> GSHMAITGTIAAIATAIVPQQGSVGIVRVSGSQAIAIAQTLFDAPGKQVWESHRILYGYIRHPQTRQIVDEALLLLMKAPRSYTREDVVEFHCHGGIIAVQQVLQLCLESGARLAQPGEFT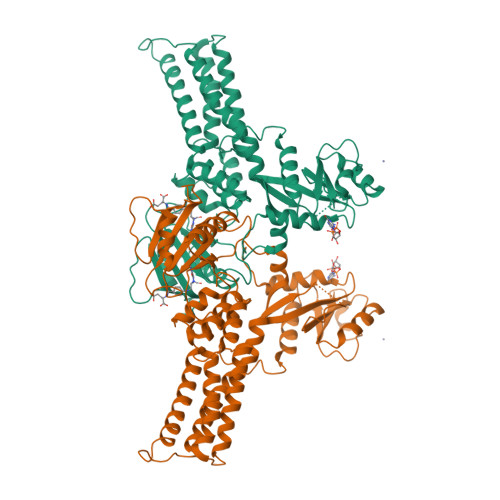LRAFLNGRLDLTQAESIADLVGARSPQAAQTALAGLQGKLAHPIRQLRANCLDILAEIEARIDFEEDLPPLDDEAIISDIENIAAEISQLLATKDKGELLRTGLKVAIVGRPNVGKSSLLNAWSQSDRAIVTDLPGTTRDVVESQLVVGGIPVQVLDTAGIRETSDQVEKIGVERSRQAANTADLVLLTIDAATGWTTGDQEIYEQVKHRPLILVMNKIDLVEKQLITSLEYPENITQIVHTAAAQKQGIDSLETAILEIVQTGKVQAADMDLAINQRQAAALTQAKMSLEQVQATITQQLPLDFWTIDLRGAIQALGEITGEEVTESVLDRIFSRFCIGK>MSPLKNLVLDIDYNDAVVVIHTSPGAAQLIARLLDSLGKAEGILGTIAGDDTIFTTPAN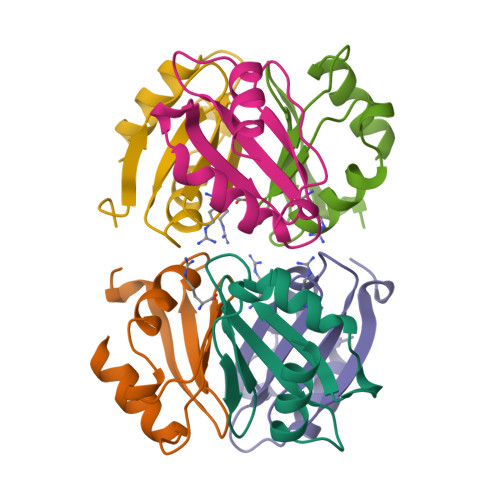GFTVKDLYEAILELFDQEL[6x]Copper-containing nitrite reductases (CuNiRs) catalyse the one-electron reduction of nitrite to nitric oxide: NO2−+2H++e− ↔ NO+H2O, a step in the microbial ATP-generating respiratory dentrification pathway. CuNiRs are trimeric and each monomer has two characteristic β-sandwich cupredoxin domains that contain a T1Cu centre with (Cys–Met–His2) ligation. The active site is a T2Cu with (His3–H2O) ligation, which is situated at the interface between two adjacent monomers in a cleft ~12 Å from the protein surface. Electrons produced during denitrification are donated to the T1Cu site by a partner redox protein and subsequently transferred via a 12.6-Å His–Cys bridge to the T2Cu centre in a proton-gated reaction.

Here we show that substitution of a surface residue (F306C) at the entrance of the channel of CuNiR results in an altered second sphere coordination of the active site Cu. Comparison of the crystallographic structures of the ‘as isolated’ (1.7 Å resolution) and substrate bound (1.75 Å resolution), allowed us to assess the effect of this substitution on the substrate access channel and its associated water network. Access to the active site from bulk solvent was also improved, as illustrated by the ability of nitrite to diffuse into the T2Cu active site in the crystal despite polyethylene glycol molecule (PEG) (present as a component of the crystallization medium) being bound across the mouth of the substrate channel. Previously, we have shown that the T2 site is not accessible to nitrite in crystals of wild-type AxNiR where PEG effectively blocks the channel. The binding of nitrite to the T2Cu results in Met135 adopting largely an ‘open’ conformation across the substrate access channel, suggesting a communication linkage between the substrate-bound T2Cu and the distant Met135. In fact, this change has been observed in the wild-type AxNiR enzyme and several other CuNiRs upon nitrite binding but its significance had remained unnoticed. The effects of surface residue substitution, F306, described here produce sufficient flexibility to allow increased solvent/substrate access, illustrated by the presence of a second water molecule (W2) in the active site pocket and also improved access to nitrite since binding is not prevented by PEG bound at the channel’s entrance. However, the substitution of F306 resulted in an approximately fourfold increase in specific activity and had a marked effect on the apparent KM for nitrite, which with a value of 1.2±0.1 mM is some 50-fold weaker than for wild-type AxNiR. The apparent affinity for nitrite obtained from the laser flash-photolysis data (Ks=0.8±0.1 mM) is in the same range as the apparent KM value obtained from the steady-state activity (KM=1.2±0.1 mM).

> DADKLPHTKVTLVAPPQVHPHEQATKSGPKVVEFTMTIEEKKMVIDDKGTTLQAMTFNGSMPGPTLVVHEGDYVQLTLVNPATNAMPHNVDFHGATGALGGAKLTNVNPGEQATLRFKADRSGTFVYHCAPEGMVPWHVVSGMSGTLMVLPRDGLKDPQGKPLHYDRAYTIGEFDLYIPKGPDGKYKDYATLAESYGDTVQVMRTLTPSHIVFNGKVGALTGANALTAKVGETVLLIHSQANRDTRPHLIGGHGDWVWETGKFANPPQRDLETWFIRGGSAGAALYTFKQPGVYAYLNHNLIEACELGAAGHIKVEGKWNDDLMKQIKAPAPIPR>[4x]MAHHHHHHMDIVSVALKRYSTKAFDATKKLTAGEAEQLKTLLQYSPSSTNSQPWHFIVASTDEGKARVAKAASGTYVFNERKILDASHVVVFCAKTAMDDAWLQRVVDQEEADGRFA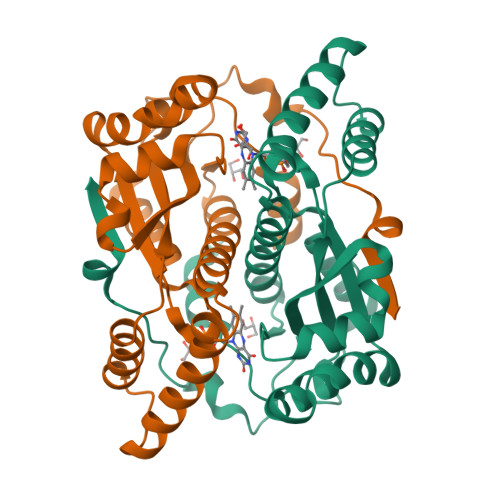TPDAKAANHKGRTFFADMHRKELKDDDQWMAKQVYLNVGNFLLGVAAMGLDAVPIEGVDFAILDEEFDLKAQGYTSLVVVPVGHHSAEDFNATLPKSRLPQSTTITEI>[26x]MSNMEKHLFNLKFAAKELSRSAKKCDKEEKAEKAKIEKAIQKGNMEVARIHAENAIRQKNQAVNFLRMSARVDAVAARVQTAVTMGKVTKSMAGVVKSMDATLKTMNLEKISALMDKFEHQ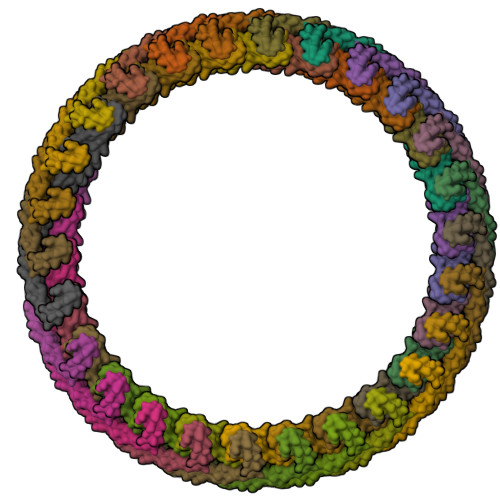FETLDVQTQQMEDTMSSTTTLTTPQNQVDMLLQEMADEAGLDLNMELPQGQTGSVGTSVASAEQDELSQRLARLRDQV> AMEQEAVSQLPTIHTKATQEESLKVDQSANSKFVAPLLDTPKSVSVISKQLIEDTKVTTLADALRTVPGITLGAGEGGNPNGDRPFIRGYSSESSMYIDGIRNSTSQNREMFAVEQVEVTKGSASAMGG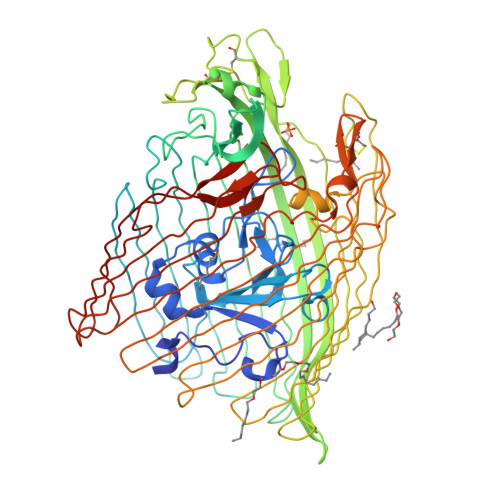AGSVGGSINMISKVAKKGDFLEGSVAAGTDNYQRITLDGNKDFGNGIAARVAVLGHQNEKAGQSNGAEYKRVGIAPSITFGLDTPTRATLSYYYLQTDDKPDSGIPYWDSSLGKAQGKPAEVKQGTYYGWKDRDFQKQENHIGTIKLEHDLTDNITITNTAMYAKSKNDYVWTNPDDSKGNVGKGLVWHRLNSAITDSETFTDQLALTGKFDTGFLKHRFNVGAEYSKQKTDKGGYNIIDAKGNVSSTGFYSDCSDLSTNWCTSLNGPTQKPFVDRLQARPDFDATVESTSVYLLDNIEITPKWLLDLGLRWDKFEAEQNFLATSSAAAYTAKNNSDFVTYQAGITFKPTENGSIYTSYATSASPVGLNAGWGDNSETINANNQMIDPEEAQTFEIGTKWDFLDNHLNLTAAIFRTEKQNTRVQIDPTTYANVGESKVDGFELGLNGEITDKWNISAGYTYLDSELTKNGKSCRSGKCTDQSIYNGNQMPNVPKQAATLWTTYKVLPQLTVGAGAVYSDKVYGDVANTKWVPSYVRYDAMARYNVNKNVDLQLNINNLSDKRYFTKAYASHYATEAEGRSAVLAVNFKY>[2x]EEEEL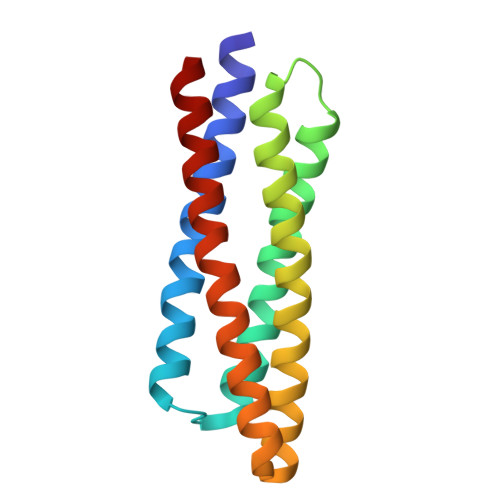EELAKELEKILRDEEGHLRKLKEALAEGLGDAEEAAELFRAESIDEMKHAEELAKLLKKGGLDPELRELLEELAELELVAINQYREAAEAAAEAAENGSEEARAAAREALEEALALELDGAKLARAALEAVEKLL>[4x]MASVHGTTYELLRRQGIDTVFGNPGSNELPFLKDFPEDFRYILALQEACVVGIADGYAQASRKPAFI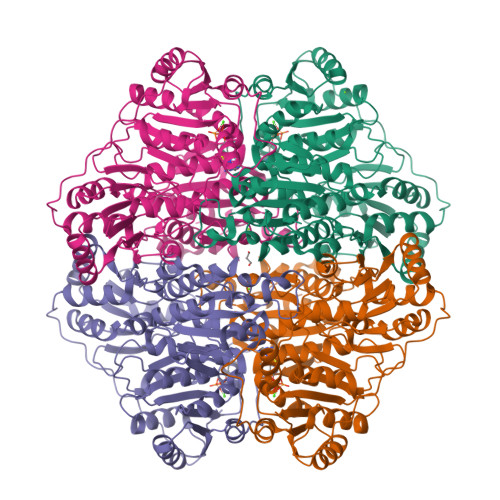NLTSAAGTGNAMGALSNAWNSHSPLIVTAGQQTRAMIGVEALLTNVDAANLPRPLVKWSYEPASAAEVPHAMSRAIHMASMAPQGPVYLSVPYDDWDKDADPQSHHLFDRHVSSSVRLNDQDLDILVKALNSASNPAIVLGPDVDAANANADCVMLAERLKAPVWVAPSAPRCPFPTRHPCFRGLMPAGIAAISQLLEGHDVVLVIGAPVFRYHQYDPGQYLKPGTRLISVTCDPLEAARAPMGDAIVADIGAMASALANLVEESSRQLPTAAPEPAKVDQDAGRLHPETVFDTLNDMAPENAIYLNESTSTTAQMWQRLNMRNPGSYYFCAAGGLGFALPAAIGVQLAEPERQVIAVIGDGSANYSISALWTAAQYNIPTIFVIMNNGTYGALRWFAGVLEAENVPGLDVPGIDFRALAKGYGVQALKADNLEQLKGSLQEALSAKGPVLIEVSTVSPVKHHHHHH>[2x]SGH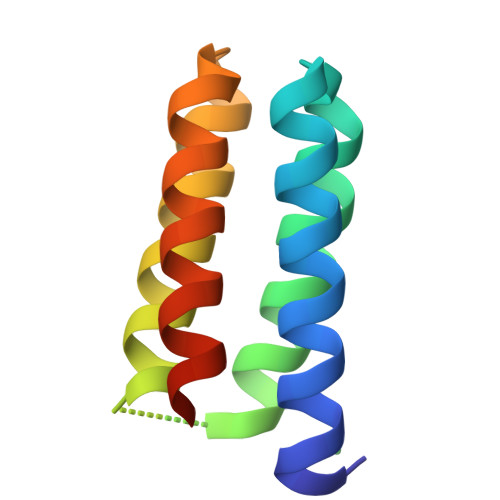TAHVDEAVKHAEEAVAHGKEGHTDQLLEHAKESLTHAKAASEAGGNTHVGHGIKHLEDAIKHGEEGHVGVATKHAQEAIEHLRASEHKSH>MGSSHHHHHHSSGLVPRGSHMASNAYTERDMLQKAADETTLKNVLVMKQAWVPYPAYTDRAAWDSLMGSNKQRLIAAGEKLLDYKWQLIPATAYLEYERTGNRKIMEVPYDANRQALNTLMLAELAEGKGRFIDQLLNGAYMSCEMNSWVLSAHLPRQSSKRSLPDFREQIIDLGSGGYGALMAWVHYFFRKPFDKINPVVSLQMRKAIKERILDPYMNDDDMWWMAFNWQPGEIINNWNPWCNSNALQCFLLMENNKDRLAKAVYRSMKSVDKFINFVKSDGACEEGTSYWGHAAGKLYDYLQILSDGTGGKISLLNEPMIRRMGEYMSRSYVGNGWVVNFADASAQGGGDPLLIYRFGKAVNSNEMMHFAAYLLNGRKPYATMGNDAFRSLQSLLCCNDLAKETPKHDMPDVTWYPETEFCYMKNKNGMFVAAKGGFNNESHNHNDVGTFSLYVNTIPVILDAGVGTYTKQTFGKDRYTIWTMQSNYHNLPMINGIPQKYGQEYKATNTTCNEKKRVFSTDIAAAYPSEAKVKNWIRSYTLDDRKLTITDSYTLEEAVAPNQVNFMTWGNVTFPSQGKIQIEVKGQKVELDYPTLFKAELETIQLDDPRLSNVWGKEIYRITLKTNEKKETGNYKFVIQQIK[2x]

In bacteria, however, a different strategy employing a class of enzyme known as polysaccharide lyases (PL) is deployed. PLs selectively target glycans composed of uronic acids with a C4 hydroxyl group linked to the preceding sugar in the glycan chain. This enables PLs to operate through a β-elimination mechanism that relies on proton abstraction from the C5 carbon of the uronic acid sugar ring, resulting in double bond formation between C4 and C5 and elimination of the preceding sugar. The three characterized PL33_1 enzymes were all from Bacteroides species inhabiting the human colon: BT4410 (BtPL33HA) and BcellWH2_04512 (BcPL33HA) are hyaluronidases from Bacteroides thetaiotaomicron VPI-5482 (B. theta) and Bacteroides cellulosilyticus WH2 (B. cell), respectively, while HMPREF1181_01744 (BsPL33Heparosan) is a heparosanase from Bacteroides stercoris CC31F (B. stercoris). The enzymes are 68% identical and contain a larger N-terminal α-helical (α/α)6 toroid domain (residues 21 to 401; BtPL33HA numbering used throughout this section unless specified) and a smaller β-sheet C-terminal domain (residues 402 to 635).

Crystal structures of BtPL33HA and BcPL33HA reveal a two-domain structure. The C-terminal domain possesses an extended loop region between β-strands 5 and 6 (Leu455-Leu484: BtPL33HA, and Ile464-Leu493: BcPL33HA), forming an octahedral Zn2+ coordination site [supported by anomalous X-ray diffraction data], along with the loop region between α-helices 12 and 13 from the N-terminal domain. The two domains oppose each other in such a way that a deep, open-ended cleft is formed resembling an active site that would be compatible with an endo-processive mode of action of BtPL33HA and BcPL33HA. Analysis of the five enzymes via SEC-coupled light scattering and SAXS indicated that the three PL33_1 enzymes BtPL33HA, BcPL33HA, and BsPL33Heparosan are dimeric, while the PL33_2 enzymes ObPL33CS and ObPL33Gellan are monomeric. SAXS data indicate that the dimeric enzymes all bind as head-to-head homodimers, generating elongated envelopes. This is consistent with PISA analysis of the crystal structures of BtPL33HA and BcPL33HA which predicted a buried surface area of ~1,388 Å2 and 1,006 Å2, and a complex significance score of 0.207 and 0.290, respectively. The phenol of Y470 moves within 5 to 6 Å of the +1 GlcA and N-acetyl of the −1 GlcNAc, while F475 moves within 5 Å of the +2 GlcNAc, forming the tunnel topography. This differs significantly from the wide-open cleft observed in the crystal structures of both BtPL33HA and BcPL33HA. Fitting of both the BtPL33HA and BcPL33HA crystal structures and their AF2 models to SAXS data indicated that the best fit was for the open conformation observed in the crystal structures. Next, we performed molecular dynamic simulations to determine the extent of PL33 conformational plasticity, using the BtPL33HA crystal structure model.5-(4-bromophenyl)-~{N}-(4-piperazin-1-ylphenyl)-~{N}-(pyridin-2-ylmethyl)furan-2-carboxamide | 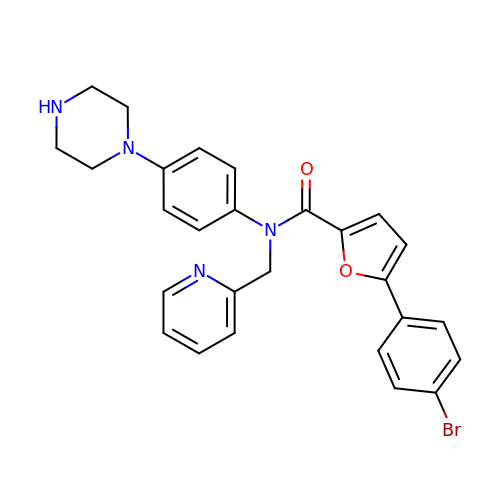C27 H25 Br N4 O2 | PCNCJMARSZPFSS-UHFFFAOYSA-N> QCDVPPNSRFDCAPDKAITQEQCEARGCCYIPAKQGLQGAQMGQPWCFFPPSYPSYKLENLSSSEMGYTATLTRTTPTFFPKDILTLRLDVMMETENRLHFTIKDPANRRYEVPLETPRVHSRAPSPLYSVEFSEEPFGVIVHRQLDGRVLLNTTVAPLFFADQFLQLSTSLPSQYITGLAEHLSPLMLSTSWTRITLWNRDLAPTPGANLYGSHPFYLALEDGGSAHGVFLLNSNAMDVVLQPSPALSWRSTGGILDVYIFLGPEPKSVVQQYLDVVGYPFMPPYWGLGFHLCRWGYSSTAITRQVVENMTRAHFPLDVQWNDLDYMDSRRDFTFNKDGFRDFPAMVQELHQGGRRYMMIVDPAISSSGPAGSYRPYDEGLRRGVFITNETGQPLIGKVWPGSTAFPDFTNPTALAWWEDMVAEFHDQVPFDGMWIDMNEPSNFIRGSEDGCPNNELENPPYVPGVVGGTLQAATICASSHQFLSTHYNLHNLYGLTEAIASHRALVKARGTRPFVISRSTFAGHGRYAGHWTGDVWSSWEQLASSVPEILQFNLLGVPLVGADVCGFLGNTSEELCVRWTQLGAFYPFMRNHNSLLSLPQEPYSFSEPAQQAMRKALTLRYALLPHLYTLFHQAHVAGETVARPLFLEFPKDSSTWTVDHQLLWGEALLITPVLQAGKAEVTGYFPLGTWYDLQTVPIEALGSLPPPPAAPREPAIHSEGQWVTLPAPLDTINVHLRAGYIIPLQGPGLTTTESRQQPMALAVALTKGGEARGELFWDDGESLEVLERGAYTQVIFLARNNTIVNELVRVTSEGAGLQLQKVTVLGVATAPQQVLSNGVPVSNFTYSPDTKVLDICVSLLMGEQFLVSWC

Retaining α-glucosidases employ a conserved two-step Koshland double displacement mechanism, in which α-glucosidase substrates are hydrolyzed using two key carboxylic acid residues functioning as the catalytic nucleophile (Asp518 in GAA and Asp412 in CjAgd31B, a bacterial homologue of GAA) and catalytic acid/base (Asp616 in GAA and Asp480 in CjAgd31B). Mutations in the gene encoding for GAA can lead to enzyme deficiency which generates multiple phenotypic forms of the lysosomal storage disorder (LSD) Pompe disease (PD). Herein, we report a 1,6-epi-cyclophellitol cyclosulfamidate as a new class of reversible α-glucosidase inhibitors that displays enzyme inhibitory activity by virtue of its conformational mimicry of the substrate when bound in the Michaelis complex.

Structural data for the rhGAA-sulfamidate 6 complex clearly revealed that the cyclosulfamidate with the oxygen attached to the pseudo-anomeric position acts as an electrophilic trap, yielding a covalent complex with the enzyme and adopting a final 1S3 conformation in the enzymatic pocket after covalent reaction with the catalytic nucleophile Asp51831. The interactions of the cyclitol moiety of sulfamidate 6 are essentially identical to those observed in the rhGAA-sulfamidate 4 complex, though the sulfamidate moiety engenders steric constraints on the active-site scaffold. The bulky sulfamidate, liberated from the cyclic restraint of the cyclophellitol framework, pushes outward Met519, Trp481, and the associated loop region. The energy cost of this structural perturbation is compensated for by several H-bonding interactions between the sulfamidate and rhGAA active-site residues, pleading for stabilization of the abortive complex. Contrary to the previously observed inactivity of the galactose-configured cyclosulfamidate analogue toward α-GalA,26 cyclosulfamidate 6 in turn proved to be an irreversible inhibitor of GAA with a KI of 378 μM and kinact of 0.35 min–1. In comparison, sulfamidate 6 with an oxygen at the pseudo-anomeric position showed to be a 10-fold less potent lysosomal GAA inhibitor, with comparable activity for the GANAB (IC50 = 112 and 47 μM, respectively). Thermostability assays (TSAs) showed that α-glc-cyclosulfamidate 4 stabilizes rhGAA with a maximum shift in inflection temperature (ΔTimax) of 11.2 °C and a half maximal effective concentration (EC50) of 1.16 μM, whereas α-glc-cyclosulfamidate 6 does not prevent enzyme unfolding at increasing temperature. Kinetic and crystallographic studies of rhGAA demonstrate that the position of the endocyclic nitrogen dictates the reactivity of these cyclic sulfamidates, and whereas cyclosulfamidate 6 reacts covalently, sulfamidate 4 binds in a competitive manner, providing a new chemical space for potential α-glucosidase stabilizers.> MSEFNEKPEKLIVDGLRLDGRKFDELRPIKIEASVLKRADGSCYLEMGKNKVIAAVFGPREVHPRHLQDPSKAIIRYRYNMAPFSVEERKRPGPDRRSIEISKVSKEAFEAVIMKELFPRSAIDIFVEVLQ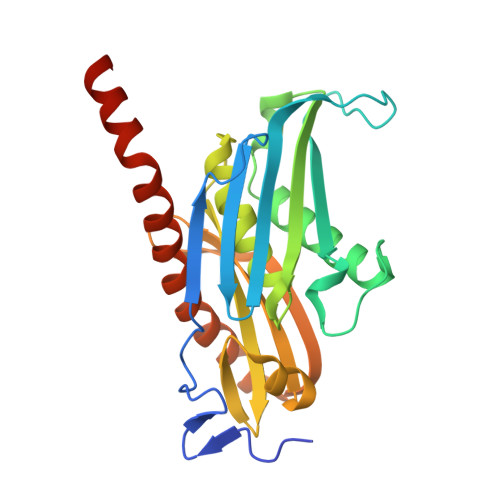ADAGSRTACLNAASVALVDAGVPMKGMITSVAVGKADGQLVLDPMKEEDNFGEADMPFAFLIRNGKIESIALLQMDGRMTRDEVKQAIELAKKGALQIYEMQREAILRRYIEVGEEMDEITEGGEDA>[8x]MGMDQQPNPPDVDAFLDSTLVGDDPALAAALAASDAAELPRIAVSAQ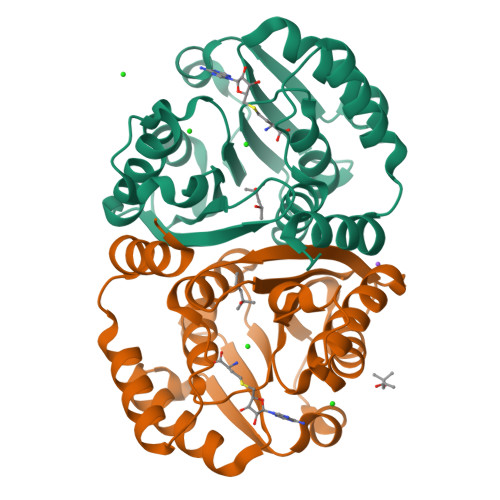QGKFLCLLAGAIQARRVLEIGTLGGFSTIWLARGAGPQGRVVTLEYQPKHAEVARVNLQRAGVADRVEVVVGPALDTLPTLAGGPFDLVFIDADKENNVAYIQWAIRLARRGAVIVVDNVIRGGGILAESDDADAVAARRTLQMMGEHPGLDATAIQTVGRKGWDGFALALVRENLYFQGGHHHHHHG4-([1,3]thiazolo[4,5-b]pyridin-2-yloxy)benzaldehyde | C13 H8 N2 O2 S | 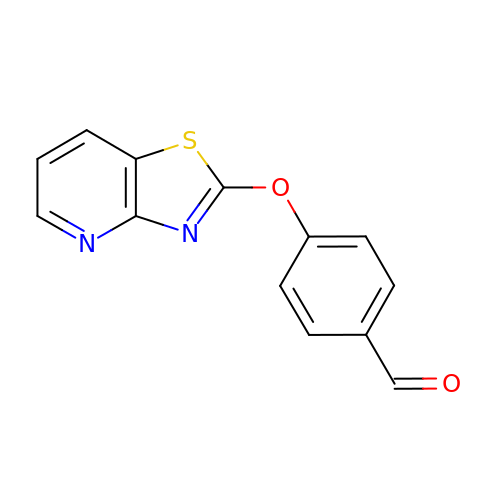MIXDMADWNWRCQX-UHFFFAOYSA-N>GAMAGKSSLFKVILLGDGGVGKSSLMNRYVTNKFDTQLFHTIGVEFLNKDLEVDGHFVTMQIWDTAGQERFRSLRTPFYRGSDCCLLTFSVDDSQSFQNLSNWKKEFIYYADVKEPESFPFVILGNKIDISERQVSTEEAQAWCRDNGDYPYFE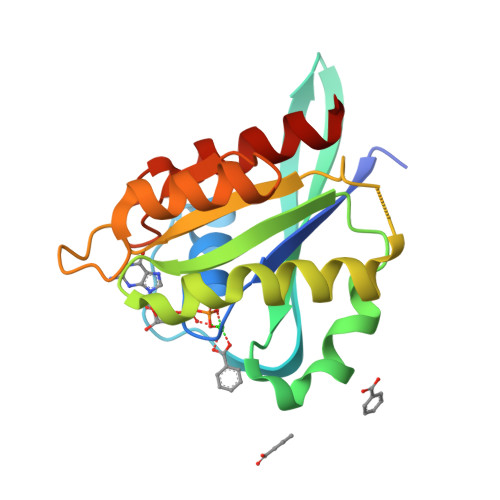TSAKDATNVAAAFEEAVRRVLAT[2x]>[5x]ASNFTQFVLVDNGGTGDVTVAPSNFANGVAEWISSNPRSQAYKVTCSVRQSSAQNRKYTIKVEVPKVATQTVGGVELPVAAWRSYLNMELTIPIFATNSDCELIV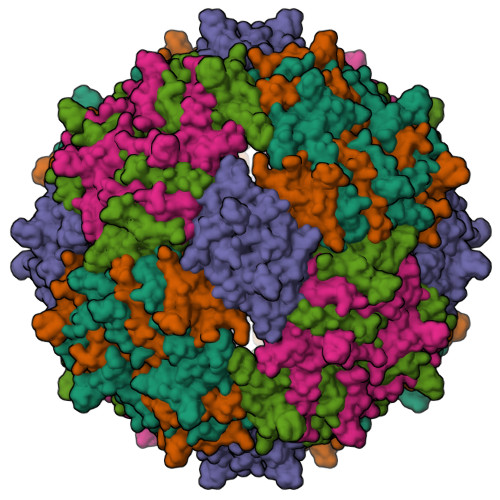KAMQGLLKDGNPIPSAIAANSGIY> MTQELGNANFENFIGATEGFSEIAYQFTSKILTLGYAVMLAGLLYFILTIKNVDKKFQMSNILSAVVMVSAFLLLYAQAQNWTSSFTFNEEVGRYFLDPSGDLFNNGYRYL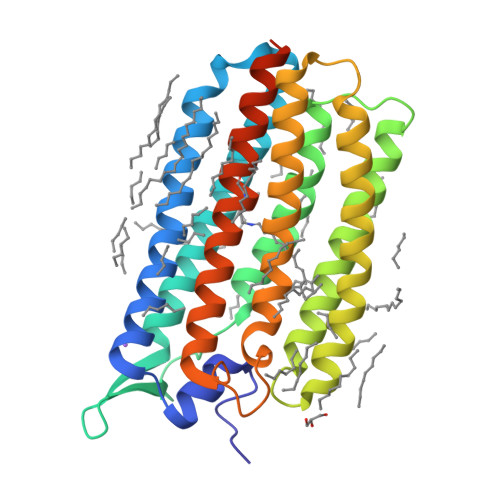NWLIDVPMLLFQILFVVSLTTSKFSSVRNQFWFSGAMMIITGYIGQFYEVSNLTAFLVWGAISSAFFFHILWVMKKVINEGKEGISPAGQKILSNIWILFLISWTLYPGAYLMPYLTGVDGFLYSEDGVMARQLVYTIADVSSKVIYGVLLGNLAITLSKNKELVEANSLEHHHHHH2-naphthalen-1-yl-1,3-thiazole-4-carboxylic 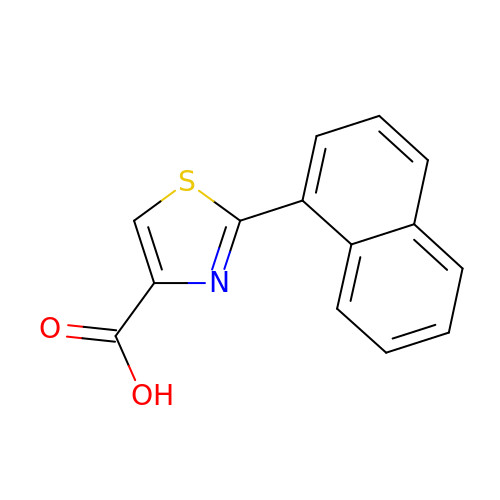acid | C14 H9 N O2 S | AQRUWPVKXHZCKR-UHFFFAOYSA-N>MIINEKYPYLSYLLRCYFNQDFEVLFGNADETLAAYKATETAEERLQMKAEIDYLLALSLPDDELQDILLNKLDCSYYYPNEWSSSEEWLKHIYKQMNHHHHHH[3x];>[3x]GGHLIDRHVGKTEAELLNRVSTGNVKSASSFTDRTTAEAVTSKAIDSNQAKIDSYLSGSQKGYLEIDYQSNVPIGISVSRGSTNVSSVTNARIIIA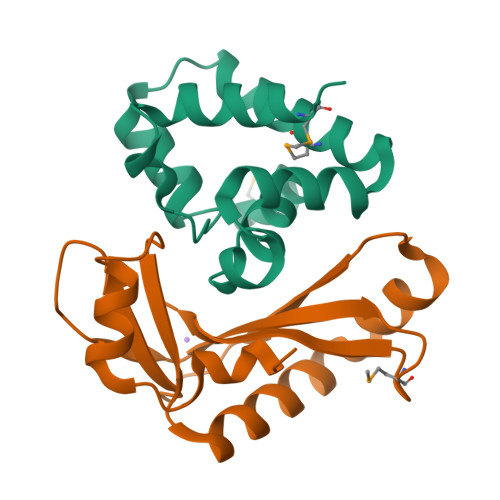RDPSMPTGYKIITGYPTP> MNQLFSQGGKGSAGILTNKQAVARHFGVKQ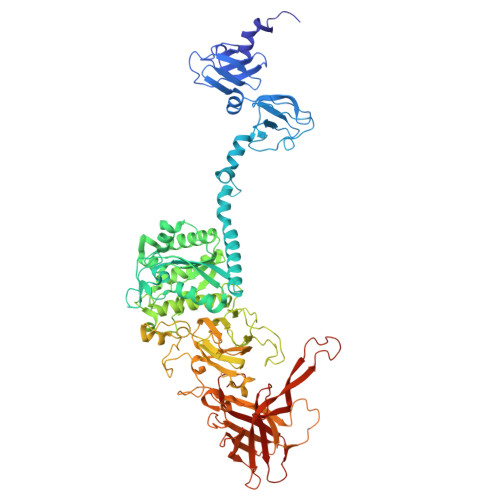SEVVYFSVGVDISGYKVIYDKTTQRAYSLPIGIPAGTTAISLSTAAVLVHSQGSVDLGAVAVLRKEYVTIPGDFTSGATIQVKNEILTHSNGAQYRWAGAVPKVVPAGSTPASSGGISASAWIEVTGEELRDELATTGGASQIGTSDGKTVQQWIIANDSANYRARNIQKLAWVDKQVHSRGSIKVLFQGDSMTAGYDTTSTDRVPANNGDWATHASMTYPQRFMAYLPEQSGCSVTGVYRAISGHTAIQSYNEPSWQSNPNCDVVILMLGLNDAGGVAGTTEDIYMEYMEKLIRRFIDWGMGVVVQTCSTGGQGSGGVVANLWAKRMRMMADTYGCAHFNADEVQYYRHNGAVQSDGGHFNSMGYAIHGQMLASMFMAGGLLPTYRPLTNEINTWCGRLDDSIGYCDATGNINLGRSDGAYTRTKVVGGMLANVASIATFSFYLDAEAAHIFVHGSGAGPINVLVDAPSWWNNGAQDYYDFANNQSINFSNSPQAANNAIVDLSTTYSADRKFVGRILGRGWKTLTFFTNLQGTGGDFYLNSLTVQPVPVGMSVQARNWARFDKGHRAVYSKKIPQAYNQATLPTATALVNFQVPMPQSMLPTTPSISGDLGTNFYNCGHSVLKISNSSGDYLEVLLIKTTGGGYVFTGKILKTTYATGNQPTAITATAAHYSMKDLKVAGANGPNMPLETIRDIDMASYVTIGVGAGNGGLVLDINITWPSTPPTSYWNIELEAWDMFGNSEASI> MKDRFELVSKYQPQGDQPKAIEKLVKGIQEGKKHQTLLGATGTGKTFTVSNLIKEVNKPTLVIAHNKTLAGQLYSEFKEFFPNNAVEYFVSYYDYYQPEAYVPQTDTFIEKDASINDEIDKLRHSATSALFERRDVIIIASVSCIYGLGSPEEYREMVVSLRTEMEIERNELLRKLVDIQYARNDIDFQRGTFRVRGDVVEIFPASRDEHCVRVEFFGDEIERIREVDALTGEILGDRDHVAIFPASHFVTRAEKMEKAIQNIEKELEEQLKVMHENGKLLEAQRLEQRTRYDLEMMREMGFCSGIENYSRHLTLRPPGSTPYTLLDYFPDDFMIVVDESHVTIPQVRGMFNGDQARKQVLVDHGFRLPSALDNRPLRFEEFEKHMHNIVYVSATPGPYEIEHTDEMVEQIIRPTGLLDPLIDVRPIEGQIDDLIGEIQARIERNERVLVTTLTKKMSEDLTDYLKEIGIKVNYLHSEIKTLERIEIIRDLRLGKYDVLVGINLLREGLDIPEVSLVAILDADKEGFLRSERSLIQTIGRAARNAEGRVIMYADKITKSMEIAINETKRRREQQERFNEEHGITPKTINKEIRDVIRATVAAEDKAEYKTKAAPKLSKMTKKERQKVVEQMEHE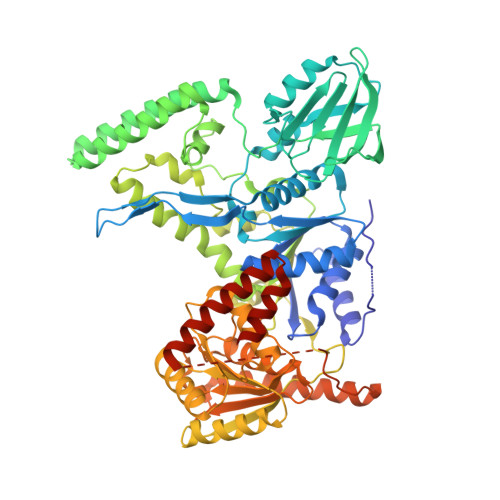MKEAAKALDFERAAELRDLLLELKAEG>MLKRVEIFTDGSCLGNPGPGGYGAILRYRG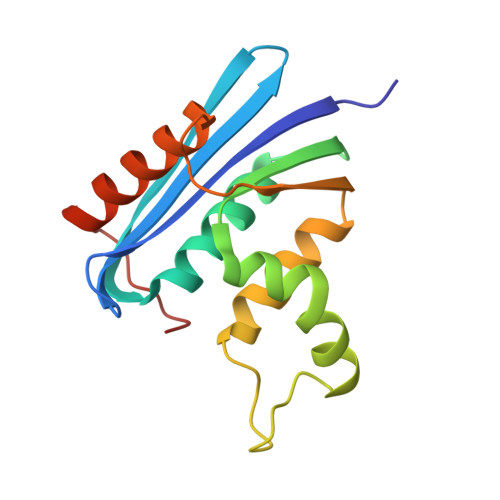REKTFSAGYERTTNNRMELMAAIVALEALKEHCEVILSTDSHYVRKGITEWIHNWKKRGWKKADKKPVKNVDLWKRLDAALGRHKIKWEWVKGHAGHPENERCDELARAAAMNPTLEDTGYQVEV[2x]>MSASIPDIKLSSGHLMPSIGFGCWKLANATAGEQVYQAIKAGYRLFDGAEDYGNEKEVGDGVKRAIDEGLVKREEIFLTSKLWNNYHDPKNVETALNKTLADLKVDYVDLFLIHFPIAFKFVPIEEKYPPGFYCGDGNNFVYEDVPILETWKALEKLVAAGKIKSIGVSNFPGALLLDLLRGATIKPAVLQVEHHPYLQQPKLIEFAQKAGVTITAYSSFGPQSFVEMNQGRALNTPTLFAHDTIKAIAAKYNKTPAEVLLRWAAQRGIAVIPKSNLPERLVQNRSF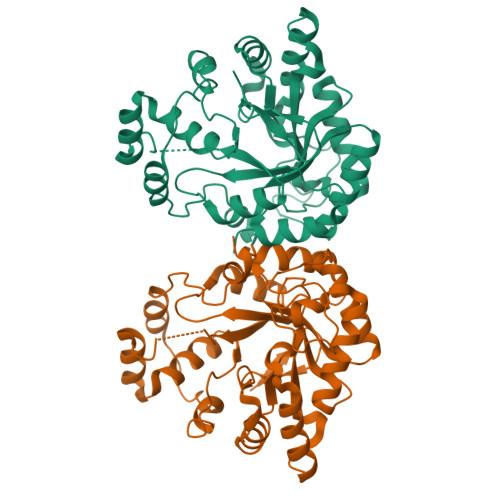NTFDLTKEDFEEIAKLDIGLRFNDPWDWDNIPIFV[2x]>[4x]MGSDKIHHHHHHVLIWWRGKFRRADEISLDFSLFEKSLQGAVYETLRTYSRAPFAAYKHYTRLKRSADFFNLPLSLSFDEFTKVLKAGADEFKQEVRIKVYLFPDSGEVLFVFSPLNIPDL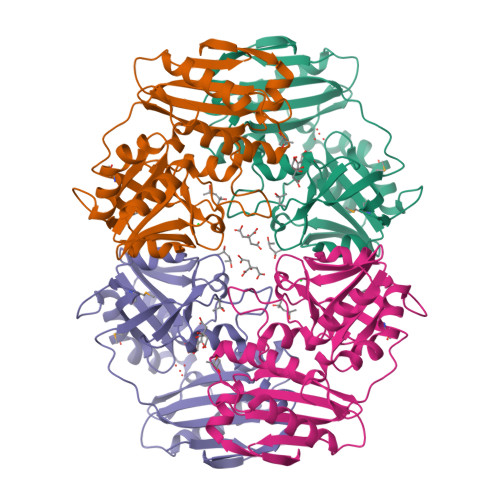ETGVEVKISNVRRIPDLSTPPALKITGRTDIVLARREIVDCYDVILLGLNGQVCEGSFSNVFLVKEGKLITPSLDSGILDGITRENVIKLAKSLEIPVEERVVWVWELFEADEMFLTHTSAGVVPVRRLNEHSFFEEEPGPVTATLMENFEPFVLNLEENWVGI>SMKFQARVLTLYPEMFPGFLGCSLAGQALKQGIWSLETVQIRDFALDKHHSVDDTPAGGGAGMVMRADVLAAALDSCPNDSPRLLMSPRGRLLNQAYARSLARSSGVTLVCGRFEGVDERIIEARELEEVSIGDYILSGGETAALVLLDAIVRLLPGVMGNEISAKCESFENGLLEHPQYTRPAVFEGRGIP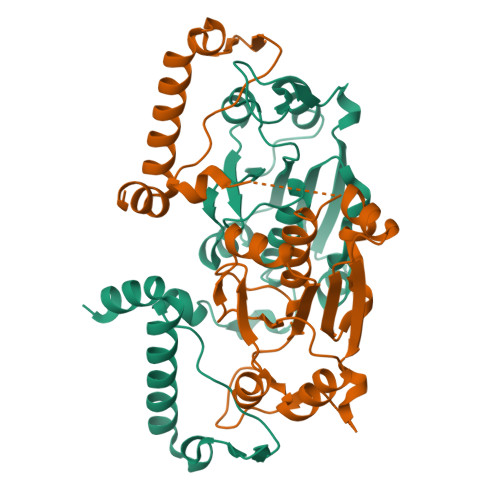PVLTSGHHKAIANWRQQQAESLTRQRRPDLYALYNKNRQKT[2x]> GMGYNTIPAGKDLPNDIYVAIEIPANASPIKYEIDKDMDALLVDRFMATPMFYPANYGYINNTLADDGDALDVLVITPYPVAPGSVIRARPVGVLKMSDEAG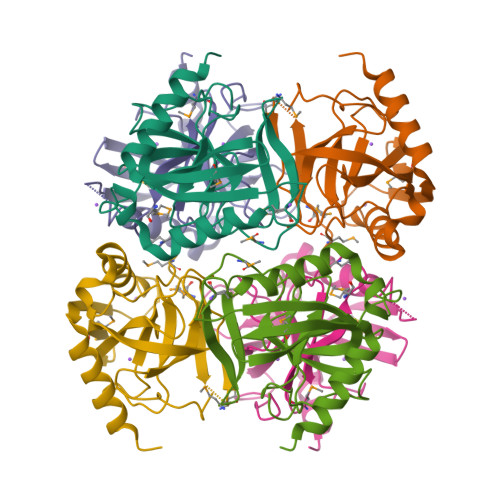GDEKLLAVPHEKLTQLYNDIHDIDDVPQLLKDQIVHFFEHYKDLEKGKWVKVEGWENADAARAAIVKSAAAYKG> MNFNVGV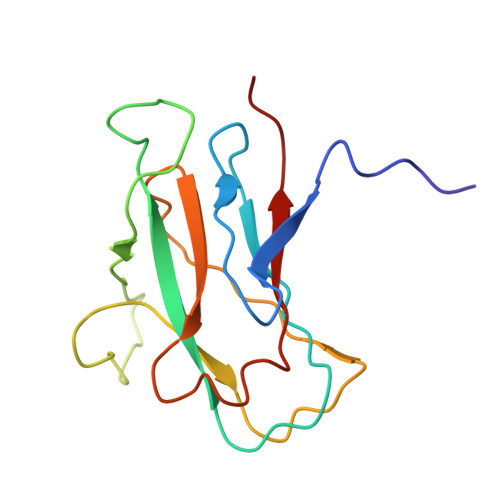DFPSFIAWDGEESFPVKVDGFNQFGFTFKTIAALTAATTFNIFYHEPSDADPCVPGPAIRVPEVPFCDTVLLSEDGLAAVTLPETVTPDSFCAGTVPCMNGQWISIAPATGSETNAANVQITVTMKGATR N-(3-methylbutanoyl)-L-valyl-N-{(1R)-1-[(R)-(2-ethoxy-2-oxoethyl)(hydroxy)phosphoryl]-3-methylbutyl}-L-valinamide 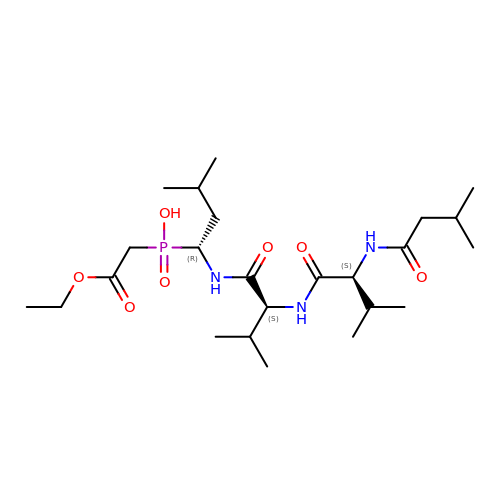| C24 H46 N3 O7 P | GSDBAIBPJKAZKN-HJNYFJLDSA-N The 2H phosphoesterase superfamily is an ancient group of proteins and protein domains characterized by a common fold and a few conserved active site residues. E. coli LigT is a 20-kDa protein that exhibits 2′,3′-cyclic nucleotide 3′-phosphodiesterase and 2′-5′-ligase/phosphodiesterase activities, but the biological function of the enzyme is unknown. The LigT structure presents a typical 2H phosphoesterase fold, in which the catalytic residues reside at the beginning of strands β2 and β6. As in other 2H family members, the active site has 2-fold symmetry; this symmetry also includes the 4 water molecules at the bottom of the active site, connecting the active-site β strands through water-mediated hydrogen bonds.

We also cocrystallized the enzyme with ATP and 3′-AMP, which are neither substrates nor products. The fact that they bind the active site can imply that they may be weak inhibitors, and it can be taken as evidence of a general propensity to bind nucleotides in the active site. Two similar datasets were collected with ATP, one of which has one ATP bound to only one of the 2 monomers in the asymmetric unit. This ATP molecule probably has a partial occupancy and/or some degree of flexibility, as evidenced by residual difference electron density. The other complex has three ATP molecules for two monomers; the space group remains the same. In addition to the ligand in both active sites, another ATP in the latter crystal form is bound in the vicinity of it in one monomer; this ATP is also involved in crystal contacts. The binding of this second ATP is a strong indication of a propensity for binding further nucleotides in the active site vicinity by E. coli LigT. Residues interacting with the second ATP include Phe159 and Arg6. Again, the α-5′-phosphate of the active-site ATP is in the same location as the corresponding phosphate in NADP+, and it is similarly coordinated by Arg6, highlighting putative RNA recognition features extending from the active site.

>GMSEPQRLFFAIDLPAEIREQIIHWRAKHFPPEAGRPVAADNLHLTLAFLGEVSAEKEKALSLLAGRIRQPGFTLTLDDAGQWLRSRVVWLGMRQPPRGLIQLANMLRSQAARSGCFQSNRPFHPHITLLRDASEAVTIPPPGFNWSYAVTEFTLYASSFARGRTRYTPLKRWALTQ[2x]We investigated the roles of three conserved prolines at positions 107, 226, and 258 in the β‐lactamase BlaC from Mycobacterium tuberculosis and found that mutations can lead to dimerization of the enzyme and an overall less stable protein that is prone to aggregate over time. BlaC has 15 proline residues but only these three are 97%–99% conserved among class A β‐lactamases (Armon et al., 2001; Ashkenazy et al., 2010; Berezin et al., 2004). In this study, we investigated the effects of substitutions on the structure, activity, and stability of BlaC. It was found that substitutions in all three prolines lead to an overall less stable enzyme, more prone to oligomerization and aggregation. We propose that one of the roles of conserved prolines in BlaC is to prevent protein association and maintain the monomeric state.

Pro107 is found at the edge of a small loop, which carries the so‐called gatekeeper residue Ile105, important for substrate specificity (Feiler et al., 2013). The crystal structure of BlaC P107T was solved at 1.9 Å with an asymmetric unit comprising four molecules forming two sets of dimers. Overall, the mutant structure resembles the structure of the wild type with an average Cα RMSD of 0.28 Å, excluding the disordered region. However, large differences are present near mutation site. The region around the mutation (residues 94–117), including α‐helices 4 and 5, are restructured. Eleven residues (101–111), could not be solved due to disorder. The space normally filled by α‐helices 4 and 5 in the structure of the wild‐type enzyme is occupied by α‐helices 6 and 7 of the other molecule of the dimer pair. Residues 94–100 and 112–117 interact with each other within one enzyme molecule and with the same stretches in another enzyme molecule, forming an anti‐parallel β‐sheet and stabilizing the dimer. The dimer formation resembles domain swapping, as the region containing two α‐helices in one protein molecules gets rearranged and the space gets occupied by α‐helices of a second protein molecule. Interestingly, the crystals were formed in 50:50 ratio of phosphate buffer with pH 6.4 and malonic acid buffer with the same pH, proving that the formation of dimers is not only occurring at pH >7.5, as was observed in solution.

>[4x]DLADRFAELERRYDARLGVYVPATGTTAAIEYRADERFAFCSTFKAPLVAAVLHQNPLTHLDKLITYTSDDIRSISTVAQQHVQTGMTIGQLCDAAIRYSDGTAANLLLADLGGPGGGTAAFTGYLRSLGDTVSRLDAEEPELNRDPPGDERDTTTPHAIALVLQQLVLGNALPPDKRALLTDWMARNTTGAKRIRAGFPADWKVIDKTGTGDYGRANDIAVVWSPTGVPYVVAVMSDRAGGGYDAEPREALLAEAATCVAGVLA>MASWSHPQFEKGAVTSLYKKAGFSDKYYRSAYMNVDLNAVASNFKVFSTLHPNKTVMAVVKANAYGLGSVKVARHLMENGATFFAVATLDEAIELRMHGITAKILVLGVLPAKDIDKAIQHRVALTVPSKQWLKEAIKNISGEQEKKLWLHIKLDTGMGRLGIKDTNTYQEVIEIIQQYEQLVFEGVFTHFACADEPGDMTTEQYQRFKDMVNEAIKPEYIHCQNSAGSLLMDCQFCNAIRPGISLYGYYPSEYVQQKVKVHLKPSVQLIANVVQTKTLQAGESVSYGATYTATDPTTIALLPIGYADGYLRIM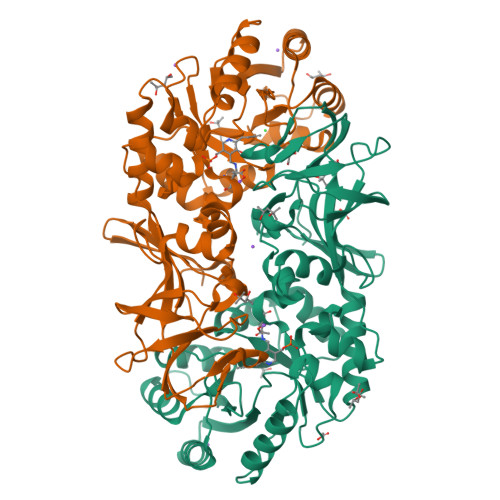QGSFVNVNGHQCEVIGRVCMDQTIVKVPDQVKAGDSVILIDNHRESPQSVEVVAEKQHTINYEVLCNLSRRLPRIYHDGDQRFVTNELLK[2x]N-prop-2-en-1-ylthioformamide | C4 H7 N S | 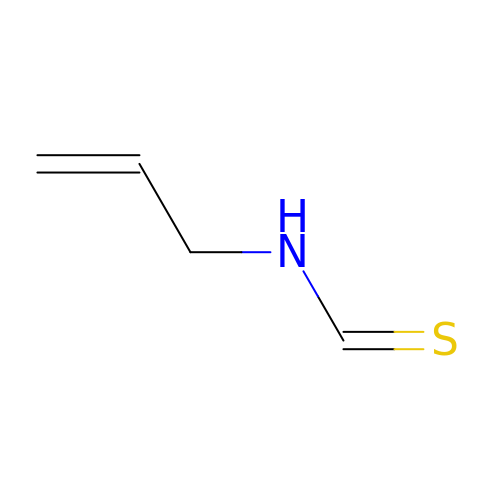PDIXEKZHQJNVMI-UHFFFAOYSA-N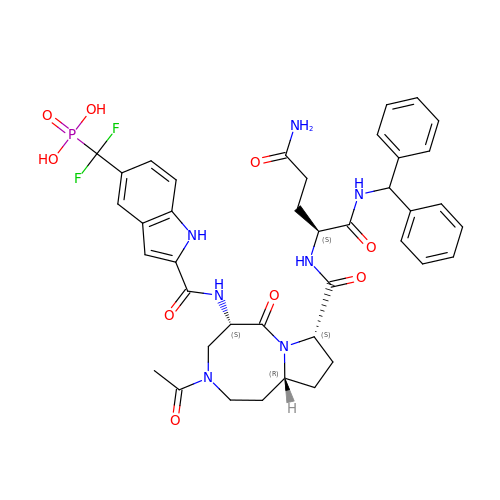[(2-{[(5S,8S,10aR)-3-acetyl-8-({(2S)-5-amino-1-[(diphenylmethyl)amino]-1,5-dioxopentan-2-yl}carbamoyl)-6-oxodecahydropyrrolo[1,2-a][1,5]diazocin-5-yl]carbamoyl}-1H-indol-5-yl)(difluoro)methyl]phosphonic acid (non-preferred name) | C40 H44 F2 N7 O9 P | HBICZHLVBCLHSV-VUCLUUCHSA-N>[8x]MSIAESSVPIAVPVPTGGDDPTKVAMLGLTFDDVLLLPAASDVVPATADTSSQLTKRIRLRVPLVSSAMDTVTESRMAIAMARAGGMGVLHRNLPVAEQAGQVETVKRSEAGMVTDPVTCSPDNTLAEVDAMCARFRISGLPVVDDTGELVGIITNRDMRFEVDQSKPVSEVMTKAPLITAKEGVSAEAALGLLRRHKIEKLPIVDGHGKLTGLITVKDFVKTEQFPLSTKDSDGRLLVGAAVGVGDDAWTRAMTLVDAGVDVLIVDTAHAHNRGVLDMVSRLKQAVGERVDVVGGNVATRAAAAALVEAGADAVKVGVGPGSICTTRVVAGVGAPQITAILEAVAACKPYGVPVIADGGLQYSGDIAKALAAGASTAMLGSLLAGTAESPGELIFVNGKQFKSYRGMGSLGAMQGRGAAKSYSKDRYFQDDVLSEDKLVPEGIEGRVPFRGPLGTVIHQLTGGLRAAMGYTGSATIEQLQQAQFVQITAAGLKESHPHDITMTVEAPNYYTR

Central to the purine metabolic pathway is inosine-5′-monophosphate dehydrogenase (IMPDH; EC 1.1.1.205), a rate-limiting enzyme catalyzing the NAD+-dependent oxidation of inosine-5′-monophosphate (IMP) to xanthosine 5′-monophosphate (XMP). Most of the IMPDHs share a conserved two-domain architecture consisting of a catalytic domain and a smaller regulatory cystathionine β-synthase (CBS) domain (also known as the Bateman module). The CBS domain serves as an allosteric regulatory module responding to the binding of nucleotide effectors. The enzyme is inhibited by both GTP and (p)ppGpp, which bind to the regulatory CBS domains and, via interactions with basic residues in hinge regions, lock the catalytic core domains in a compressed conformation.

Surprisingly, in our study, the addition of ATP under cryo-EM conditions failed to induce the extended conformation of the MsmIMPDH octamers. The datasets of MsmIMPDH apo and ATP-bound states were homogeneous, yielding only one major 3D class (Supplementary Figs. EM-2, 4). While the CBS domains in the apo form were not resolved at all, the CBS domains in the ATP-bound form established a defined position with respect to the catalytic core. The apo MsmIMPDH showed a notably increased deuterium uptake in the region of the flap loop, the C-terminus, and the CBS domain relative to the other parts of the protein. The highly dynamic nature of these regions correlates with the drop we observed in the local resolution of the same regions and the absence of the CBS domain in the cryo-EM map in the apo form. We demonstrate that in the apo form of MsmIMPDH, the flap and finger loops, which are constituents of the active site of the catalytic domains, form a packed tetramer–tetramer interface, which brings the two tetramers close together. Thus, the two tetramers adopt predominantly a compressed inactive octameric conformation, that reduces the affinity for substrate IMP.(2~{R},4~{R})-4-fluoranyl-1-[1-(4-methoxyphenyl)cyclohexyl]carbonyl-~{N}-(1~{H}-pyrazolo[4,3-b]pyridin-5-yl)pyrrolidine-2-carboxamide 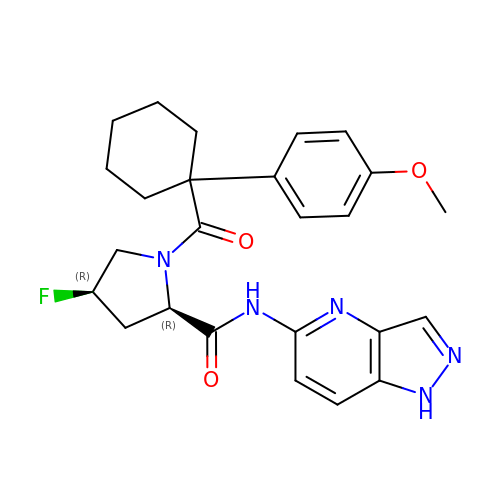| C25 H28 F N5 O3 | CCRMEUSDGNVQDG-DYESRHJHSA-N>[4x]GIDPFTATIARKGEGSVLEQIDQGSILKLPSNLLFENATSDAINQDMMLYIERIAKIIQKLPKRVHINVRGFTDDTPLVKTRFKSHYELAANRAYRVMKVLIQYGV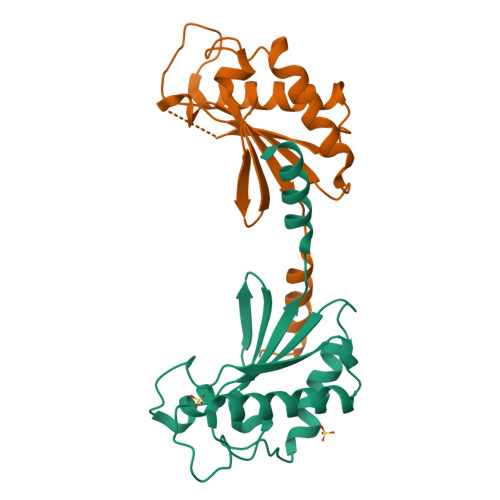NPNQLSFSSYGSTNPIAPNDSLENRMKNNRVEIFFSTDANDLSKIHSILDNEFNPHKQQE In the Firmicute B. subtilis, the ytqI gene product was shown to be a major nanoRNA turnover enzyme, and was renamed NanoRNase A (NrnA). We show here that Bacillus NrnA is a bidirectional nuclease that can degrade RNA fragments from either the 3′ or the 5′ end. We have determined crystal structures of B. subtilis NrnA in its apo form, as well as complexed with substrates. These structures reveal a dynamic bi-lobed molecule with the DHH catalytic domain and the DHHA1 substrate binding domains connected through an extended linker.

In the crystals of NrnA H103A soaked with both MnCl2 and pAp, electron density corresponding to the full pAp ligand is not seen, presumably because the mutant still retains some residual activity. Instead, additional tetrahedral electron density outside M2 is clearly visible in all four chains when 2Fo-Fc and Fo-Fc electron density maps are contoured at 1.75 σ and 3.50 σ respectively. Strong 2Fo-Fc electron density (ranging from 9.0 σ to 6.5 σ) was seen at two positions in each active site for all four molecules in the asymmetric unit. This density was modeled as two Mn2+ ions present at full occupancy. Two bound Mn2+ ions at the NrnA active site are characteristic of DHH family active sites including those of inorganic PPase and RecJ, as well as NrnA homologs. Metal 2 (M2) also coordinates with aspartate carboxylates including of D24, as well as a histidine, H20, which is substituted by an Asp in the RecJ active site. A difference map contoured at 5.0 σ revealed the presence of an ordered water molecule between M1 and M2 that provides additional oxygen ligands to the metal ions and may be activated for nucleophilic attack of the incoming substrate. H104, the second histidine in the signature DHH motif, does not coordinate with M2 and is therefore accessible for interaction with the substrate’s phosphodiester backbone. We can take the product phosphate seen at the active site in our H103A:Mn:pAp structure, the 3′ nucleotide from the H103A:pAp structure, and the planar density outside F162 observed in the H103A:pAA*A to build a composite model of the pApA dinucleotide in the B. subtilis NrnA active site.

>MGSSHHHHHHENLYFQSMASMKTELIRTISLYDTIILHRHVRPDPDAYGSQCGLTEILRETYPEKNIFAVGTPEPSLSFLYSLDEVDNETYEGALVIVCDTANQERIDDQRYPSGAKLMKIDAHPNEDPYGDLLWVDTSASSVSEMIYELYLEGKEHGWKLNTKAAELIYAGIVGDTGRFLFPNTTEKTLKYAGELIQYPFSSSELFNQLYETKLNVVKLNGFIFQNVSLSENGAASVFIKKDTLEKFGTTASEASQLVGTLGNISGIRAWVFFVEEDDQIRVRFRSKGPVINGLARKYNGGGHPLASGASIYSWDEADRILADLETLCKEHE[4x]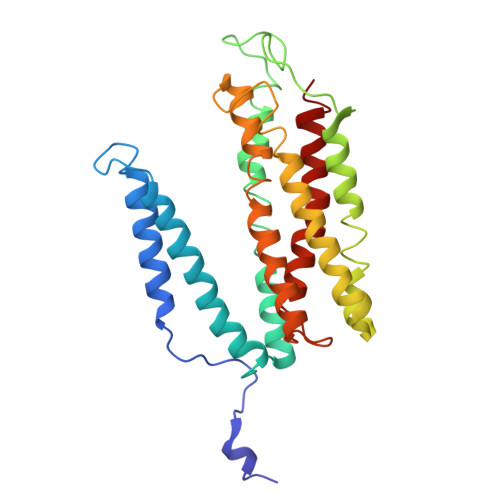> THLERSRHQQHPFHMVMPSPWPIVVSFALLSLALSTALTMHGYIGNMNMVYLALFVLLTSSILWFRDIVAEATYLGDHTMAVRKGINLGFLMFVLSEVLIFAGLFWAYFHSAMSPDVTLGACWPPVGIEAVQPTELPLLNTIILLSSGATVTYSHHALIAGNRNKALSGLLITFWLIVIFVTCQYIEYTNAAFTISDGVYGSVFYAGTGLHFLHMVMLAAMLGVNYWRMRNYHLTAGHHVGYETTIIYTHVLDVIWLFLYVVFYWWGV>[2x]GAMAIRTSELLKRPPVSLPETATIREVATELAKNRVGLAVLTARDNPKRPVAVVSERDILRAVAQRLDLDGPAMPIANSPITVLDTDPVHVAAEKMRRHNIRHVVVVN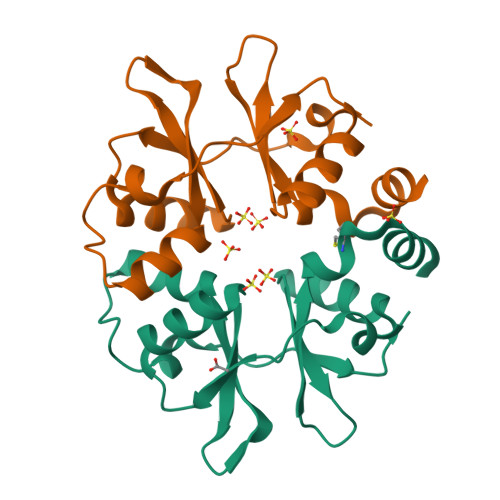KNGELVGVLSIRDLCFERAILLELATAEVPATP2-acetamido-2-deoxy-1-O-(propylcarbamoyl)-alpha-D-glucopyranose 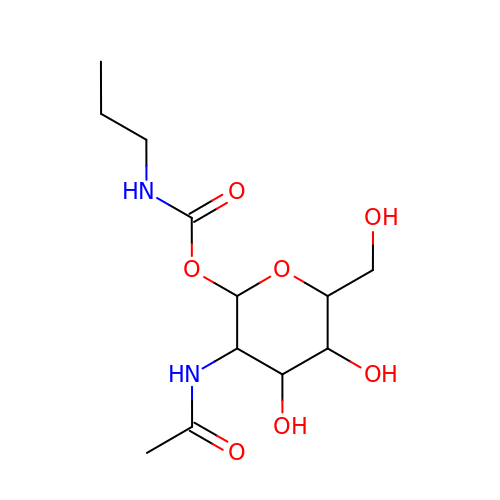| C12 H22 N2 O7 | WEAGJSCGQDTQRE-ISUQUUIWSA-N>MSDSSQLHKVAQRANRMLNVLTEQVQLQKDELHANEFYQVYAKAALAKLPLLTRANVDYAVSEMEEKGYVFDKRPAGSSMKYAMSIQNIIDIYEHRGVPKYRDRYSEAYVIFISNLKGGVSKTVSTVSLAHAMRAHPHLLMEDLRILVIDLDPQSSATMFLSHKHSIGIVNATSAQAMLQNVSREELLEEFIVPSVVPGVDVMPASIDDAFIASDWRELCNEHLPGQNIHAVLKENVIDKLKSDYDFILVDSGPHLDAFLKNALASANILFTPLPPATVDFH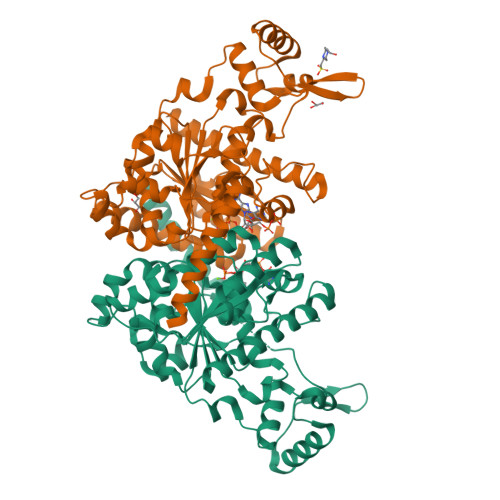SSLKYVARLPELVKLISDEGCECQLATNIGFMSKLSNKADHKYCHSLAKEVFGGDMLDVFLPRLDGFERCGESFDTVISANPATYVGSADALKNARIAAEDFAKAVFDRIEFIRSN[2x]>[12x]MEEIIVRGGNQLNGTVRIEGAKNAVLPILAASLLAEEGITTLDNVPILS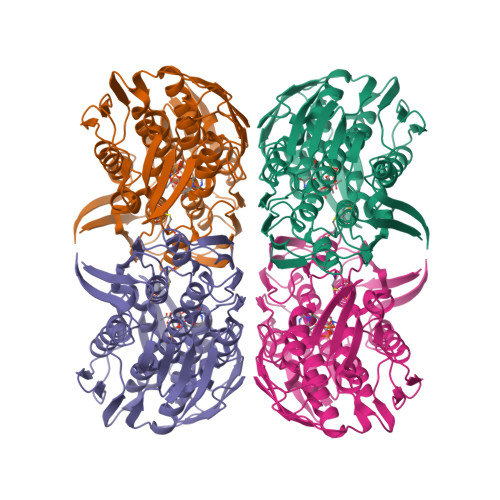DVFTMNQVIRHLNVDVDFDEQKNQVTIDASRQLEIEAPYEYVSQMRASIVVMGPLLARNGHAKVAMPGGCAIGKRPIDLHLKGFQALGAKIIQKNGYIEAIADELIGNTIYLDFPSVGATQNIMMAAVKAKGTTIIENVAREPEIVDLANILNKMGAQVYGAGTETMRIEGVDHLHAVNHSIVQDRIEAGTFMVAAAMTQGNVLIADAISEHNRPLISKLIEMGAEIIEEEGGVRVIGPKHILPTDVKTMPHPGFPTDMQAQMTAIQLVAEGTSVVTETVFENRFQHLEEMRRMNAHVKIDGNVAIMDGNHELQGAEVYATDLRAAAALVLAGLKANGITRVRNLNYLDRGYYNFHIKLQQLGADVERVDMDQTSAEKTAQTIA>GAMASARSLRSLQRQRAILKVMNTIGGVAYLREQFYESVSKYMGSTTTLDKKTVRGDVDLMVESEKLGARTEPVSGRKIIFLPTVGEDAIQRYILKEKDS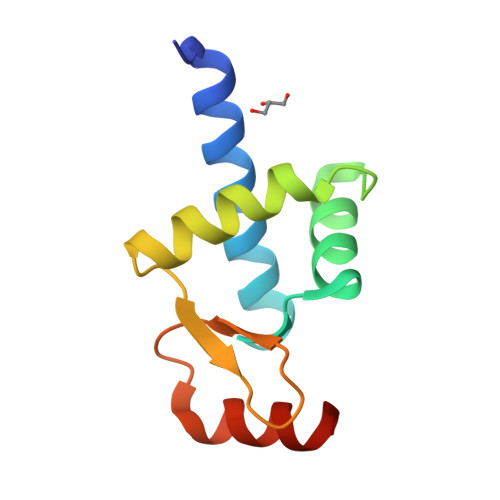[2x]Briefly, this product is produced by a typical NRPS assembly line of four subunits: PchD, PchE, PchF, and PchG. PchD activates salicylate, PchE and PchF successively integrate two l-cysteines into the growing peptide to form two thiazoline rings, and PchG then reduces the second thiazoline ring to thiazolidine before the release of mature pyochelin. The adenylation domain (A) in PchE selects and activates l-cysteine; aryl carrier protein (ArCP) and peptidyl carrier protein (PCP) connect and transfer salicylate and l-cysteine using phosphopantetheine (pPant) arms, respectively; the heterocyclization domain (Cy) condenses and cyclizes the two substrates to form a thiazoline ring; and the inserted epimerase (E) catalyzes the epimerization of an l-cysteinyl moiety to d-cysteinyl during thiazoline ring formation. The structure of PchE adopts an “H”-shaped head-to-tail dimeric architecture containing five connected catalytic domains.

In conformation 1, chains A and B are identical with an r.m.s.d. of 0.037 Å. The ArCP domains of both chains bind at the donor sites of the Cy domains, with the salicyl-pPant ligands observed, representing the substrate donation states. The Acore with interrupted Asub domains (complexed with Cys-AMP and Mg2+ ligands) are in the thioester-forming conformation but without the PCP domain captured. The E domain in this conformation may represent the epimerization conformation because the low-resolution map of the PCP domain was only observed binding to the E domain in this position (described later in Fig. 5). The tunnel surface for salicyl-pPant binding was clearly identified in the A chain of conformation 1. In particular, the D240, P370 and S448 residues are in the range for hydrogen bond formation with the pPant arm atoms, and Y114 can form a polar interaction with the thioester sulfur. The residues C129, H130, A131, L236, L471, Q473, and M470 form the salicyl moiety-binding pocket, and an additional Y484 residue forms a hydrogen bond with its hydroxyl group. These interactions position the salicyl-pPant donor in place for the condensation reaction. In the thioester-forming conformation of conformation 1_chain B, the aromatic residue F741 in the A4 motif51 was observed in two side chain conformations with a rotation angle of ~68°, similar to the H207 movement of 4CBL52 crystal structures. When the side chain of F741 points toward the active site, the pantetheine tunnel is closed, whereas the tunnel is restored to the open state when this aromatic residue rotates out of the active site, making the tunnel ready for the subsequent PCP-pPant entering.

>[2x]MDLPPDSRTALRDWLTEQLADLLGEPLADVRALADDDDLLGCGLDSIRLMYLQERLRARGSTLDFAQLAQRPCLGAWLDLLACADRLSAPATVALPTAQDRDQPFELSSVQQAYWLGRGAGEVLGNVSCHAFLEFRTRDVDPQRLAAAAECVRQRHPMLRARFLDGRQQILPTPPLSCFDLQDWRTLQVDEAERDWQALRDWRAHECLAVERGQVFLLGLVRMPGGEDRLWLSLDLLAADVESLRLLLAELGVAYLAPERLAEPPALHFADYLAHRAAQRAEAAARARDYWLERLPRLPDAPALPLACAPESIRQPRTRRLAFQLSAGESRRLERLAAQHGVTLSSVFGCAFALVLARWSESAEFLLNVPLFDRHADDPRIGEVIADFTTLLLLECRMQAGVSFAEAVKSFQRNLHGAIDHAAFPALEVLREARRQGQPRSAPVVFASNLGEEGFVPAAFRDAFGDLHDMLSQTPQVWLDHQLYRVGDGILLAWDSVVGLFPEGLPETMFEAYVGLLQRLCDSAWGQPADLPLPWAQQARRALLNGQPACATARTLHRDFFLRAAEAPDADALLYRDQRVTRGELAERALRIAGGLREAGVRPGDAVEVSLPRGPQQVAAVFGVLAAGACYVPLDIDQPPARRRLIEEAAGVCLAITEEDDPQALPPRLDVQRLLRGPALAAPVPLAPQASAYVIYTSGSTGVPKGVEVSHAAAINTIDALLDLLRVNASDRLLAVSALDFDLSVFDLFGGLGAGASLVLPAQEQARDAAAWAEAIQRHAVSLWNSAPALLEMALSLPASQADYRSLRAVLLSGDWVALDLPGRLRPRCAEGCRLHVLGGATEAGIWSNLQSVDTVPPHWRSIPYGRPLPGQAYRVVDTHGRDVPDLVVGELWIGGASLARGYRNDPELSARRFVHDAQGRWYRTGDRGRYWGDGTLEFLGRVDQQVKVRGQRIELGEVEAALCAQAGVESACAAVLGGGVASLGAVLVPRLAPRAEGSMDLPAAQPFAGLAEAEAVLTREILGALLEAPLELDDGLRRRWLDWLADSAASALPSLDEALRRLGWQAAGLTAMGNALRGLLAGEQAPAALLLDPWLAPQAVAARLPDGREALARLLEALPTPAAGERLRVAVLDTRAGLWLDQGMASLLRPGLELTLFERSRVLLDAAATRLPERIVVQALDDGLLPAEHLGRYDRVISFAALHAYEASREGLALAAALLRPQGRLLLVDLLCESPLALLGAALLDDRPLRLAELPSLLADLAAAGLAPRCLWRSERIALVEALAPGLGLDAAALQAGLEQRLPQAMRPERLWCLPSLPLNGNGKVDRRRLAESMTRALGECRHEPSAEEPLEAHEQALAECWEAVLKRPVRRREASFFSLGGDSLLATRLLAGIRERFGVRLGMADFYRQPTLAGLARHLQVQTVEIEETQLEEGVLHHHHHHLPSWSHPQFEK>[2x]CG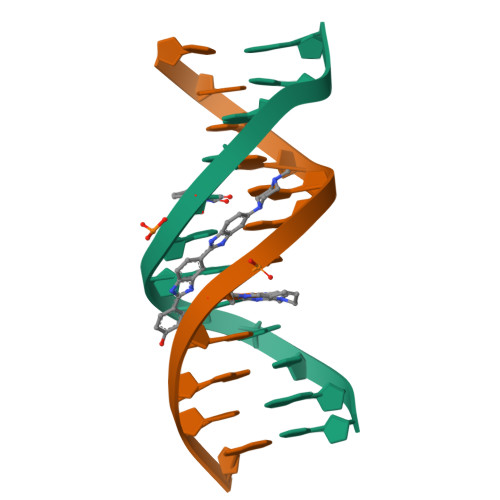CGAATXCGCG Gram-negative bacteria use type III secretion systems (T3SSs) as protein transport devices for injecting virulence effector proteins into eukaryotic cells during infection. T3SSs consist of a ‘needle complex’ (NC; Kubori et al., 1998) composed of a basal body commencing in the bacterial cytoplasm and spanning both prokaryotic membranes, into which a hollow extracellular needle is embedded that serves as secretion channel. The tip complex (TC; Mueller et al., 2005; 2008) tops the distal end of the needle. In Shigella, it is composed of two proteins, each essential to host cell sensing: IpaD and IpaB.

As wild-type TCs can exist as either homo- or heteropentamers and in order to obtain a map of the functionally relevant heteromeric tip, we used the TC map from the ΔipaB strain to remove images that contained IpaD homopentameric tips from the wild-type data set. Therefore, the one from the data set showing the lower cross-correlation should comprise primarily heteropentameric TCs. This map resolved to 24 Å resolution and also displayed a pentameric tip structure and clear helical pattern in the needle portion (left). However, the highest subunit within the wild-type map is morphologically distinct from the others and from the equivalent one in the ΔipaB map (left, thin arrows). As we have shown that IpaB (62 kDa) is found within wild-type TCs and requires IpaD (37 kDa) to localise there, we assumed that this larger subunit corresponded to IpaB. We therefore docked the cryoEM map of the needle with the lowest MxiH at the needle tip, from protofilament P1, lying right below this subunit. After subtraction of the needle density, four IpaD subunits can be docked into positions β to ε of the TC, showing that the volume occupied by the subunit in position α is larger (thin arrows). We then docked into this portion five copies of a crystal structure of IpaD that lacks its first 38 and last 10 amino acids, from which amino acids up to 125 were further removed (i.e. an IpaD fragment containing aa 126 to 322). Finally residues 323–332 were hand-built into an α-helix at the extreme C-terminus, as this region is strongly predicted to participate in IpaD's coiled coil and was not resolved in the crystal structure. However, the subunits are much further apart in the new model, allowing for the presence of both a cavity and a perpetual pore within the TC.

> GDQMISHRELWAKIANSINDINEQYLKVYEHAVSSYTQMYQDFSAVLSSLAGWISPGGNDGNSVKLQVNSLKKALEELKEKYKDKPLYPANNTVSQEQANKWLTELGGTIGKVSQKNGGYVVSINMTPIDNMLKSLDNLGGNGEVVLDNAKYQAWNAGFSAEDETMKNNLQTLVQKYSNANSIFDNLVKVLSSTISSCTDTDKLFLHF> MGSSHHHHHHSSGENLYFQGHMLRISQEALTFDDVLLIPGYSEVLPKDVSLKTRLTRGIELNIPLVSAAMDTVTEARLAIAMAQEGGIGIIHKNMGIEQQAAEVRKVKKHETAIVRDPVTVTPSTKIIELLQMAREYGFSGFPVVEQGELVGIVTGRDLRVKPNAGDTVAAIMTPKDKLVTAREGTPLEEMKAKLYENRIEKMLVVDENFYLRGLVTFRDIEKAKTYPLASKDEQGRLRVGAAVGTGADTGERVAALVAAGVDVVVVDTAHGHSKGVIERVRWVKQTFPDVQVIGGNIATAEAAKALAEAGADAVKVGIGPGSICTTRIVAGVGVPQISAIANVAAALEGTGVPLIADGGIRFSGDLAKAMVAGAYCVMMGSMFAGTEEAPGEIELFQGRSYKSYRGMGSLGAMSGSQGSSDRYFQDASAGAEKLVPEGIEGRVPYKGALSAIVHQLMGGLRAAMGYTGSADIQQMRTQPQFVRITGAGMAESHVHDVQITKEAPNYRVG

Inosine 5′-monophosphate dehydrogenase (IMPDH; EC 1.1.1.205) catalyzes the first committed reaction in de novo guanine-nucleotide biosynthesis. This enzyme converts inosine 5′-monophosphate (IMP) to xanthosine 5′-monophosphate (XMP), which can then be converted to guanosine 5′-monophosphate (GMP) by GMP synthetase. Guanine nucleotides are essential for signal transduction and DNA/RNA synthesis and IMPDH therefore plays a pivotal role in the growth and proliferation of both prokaryotic and eukaryotic cells. The enzyme mechanism is thought to start with a catalytic cysteine attacking the C2 position of IMP; an NAD+-dependent dehydro­genation then generates NADH and the covalent product intermediate E-XMP*.

Here, we report success in this endeavour and present the crystal structure of apo IMPDH from P. aeruginosa at 2.25 Å resolution. The structure is a homotetramer of subunits dominated by a (β/α)8-barrel fold, consistent with other known structures of IMPDH. Also in common with previous work, the cystathionine β-synthase domains, residues 92–204, are not present in the model owing to disorder. However, unlike the majority of available structures, clearly defined electron density exists for a loop that creates part of the active site. This loop, composed of residues 297–315, links α8 and β9 and carries the catalytic Cys304. Analysis of the Ramachandran plot revealed that 99.3% of the residues were in the allowed region, with only two outliers: Gly226 and Gln458. These two residues are located on flexible loops linking α8 to β9 and α13 to β12, respectively, and the associated electron density is relatively poor. Furthermore, PaIMPDH possesses a structural motif that indicates that this enzyme belongs to a group of IMPDHs that are susceptible to inhibitors developed to target CpIMPDH. In PaIMPDH these residues correspond to Gly19, Pro25, Thr306, Ala442, Gly445, Met393 and Glu417.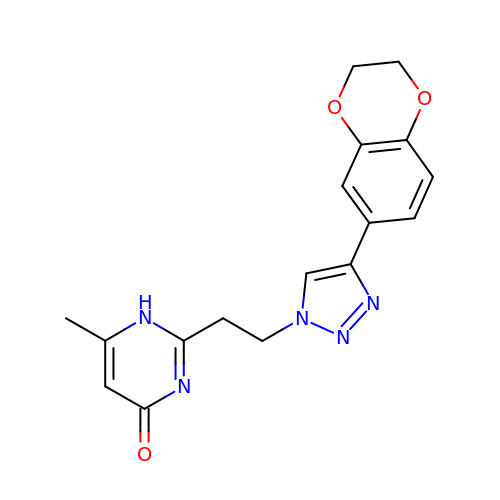2-[2-[4-(2,3-dihydro-1,4-benzodioxin-6-yl)-1,2,3-triazol-1-yl]ethyl]-6-methyl-1~{H}-pyrimidin-4-one | C17 H17 N5 O3 | HUPUXSMUAITIDA-UHFFFAOYSA-N>MATLTAKNLAKAYKGRRVVEDVSLTVNSGEIVGLLGPNGAGKTTTFYMVVGIVPRDAGNIIIDDEDISLLPLHARARRGIGYLPQEASIFRRLSVYDNLMAVLQIRDDLTSEQREDRAKELMEEFHIEHLRDSLGQALSGGERRRVEIARALAANPKFILLDEPFAGVDPISVIDIKRIIEHLRDSGLGVLITDHNVRETLAVCERAYIVSQGHLIAHGTPQQILEDEQVKRVYLGEDFRL[2x];> MIIIRYLVRETLKSQLAILFILLLIFFCQKLVRILGAAVDGDIPTNLVLSLLGLGIPEMAQLILPLSLFLGLLMTLGKLYTESEITVMHACGLSKAVLIKAAMILAVFTGAVAAVNVMWAGPWSSRHQDEVLAEAKANPGMAALAQGQFQQASDGNAVMFIESVNGNRFHDVFLAQLRPKGNARPSVVVADSGELSQQKDGSQYVTLNKGTRFEGTAMLRDFRITDFNNYQAIIGHQAVSADPDDTEQMDMRTLWKTHTDRARAELHWRFTLVATVFIMALMVVPLSVVNPRQGRVLSMLPAMLLYLVFFLLQTSIKSNGGKGKMDPAIWMWAINLLYFALAVLLNLWDTVPMRRFRARFNKGAA;> MQAFGVLDRYIGKTIFNTIMMTLFMLVSLSGIIKFVDQLKKSGQGSYDALGAGLYTILSVPKDIQIFFPMAALLGALLGLGMLAQRSELVVMQASGFTRLQVALAVMKTAIPLVLLTMAIGEWVAPQGEQMARNYRAQQMYGGSLLSTQQGLWAKDGHNFVYIERVKGNDELGGVSIYAFNPERRLQSVRYAASAKFDSENKVWRLSQVDESDLTDPKQVTGSQMVSGTWKTNLTPDKLGVVALDPDALSISGLHNYVKYLKSSGQDPGRYQLNMWSKIFQPLSVAVMMLMALSFIFGPLRSVPMGVRVVTGISFGFIFYVL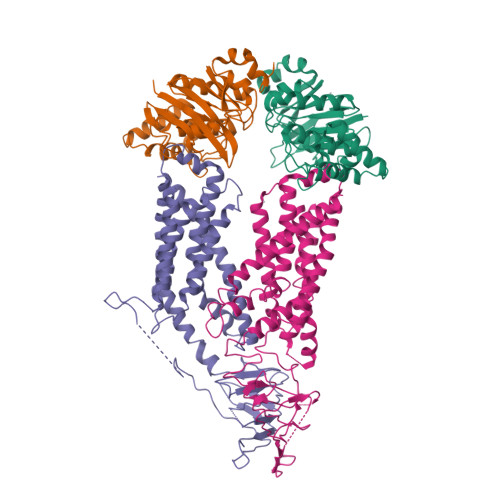DQIFGPLTLVYGIPPIIGALLPSASFFLISLWLMMRKA>MTVGYLRPTRILVDQNAIYENIQNE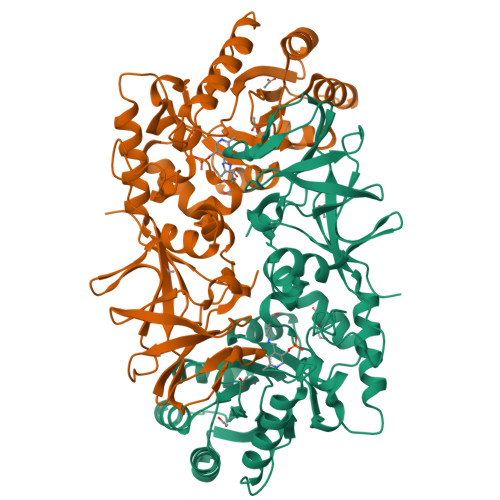LKHLEGTDTVIFPVLKANAYGHGLIPVAEVAQAAGASGFCVALLDEALALRQANFTEPILVLGITQPSEIELAAANQISLTVGSLEWLQEAAEIAQRVPYFHPLHIHLGIDSGMGRIGFRDEAELLAADAFMKAHPEYFDFEGVFTHFATADDPDDTYFKEQSARFNQLVAVLPKKPRFVHVSNSATSLWHAACNGNVIRMGISLYGLNPSGAAIPDLPYPLKPALGIESELVFVKQVAAGSKIGYGATYEASEGEWIGTIPMGYADGWLRRMSGSTVLVDGQRCEIVGRICMDQMMIRLPKRYPVGTKVVFVGKSGDDEITLQELAEYADTIHYEIICDLSDRIPRVYTGLNEH[2x]> MNLLVTSSLGVLLHLVVLCQADDHSELLVNTKSGKVMGTRVPVLSSHISAFLGIPFAEPPVGNMRFRRPEPKKPWSGVWNASTYPNNCQQYVDEQFPGFSGSEMWNPNREMSE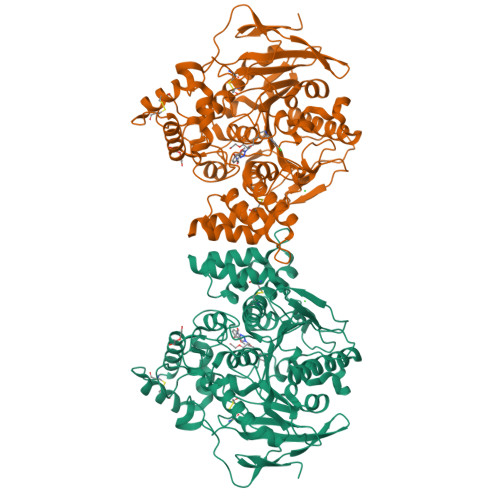DCLYLNIWVPSPRPKSTTVMVWIYGGGFYSGSSTLDVYNGKYLAYTEEVVLVSLSYRVGAFGFLALHGSQEAPGNVGLLDQRMALQWVHDNIQFFGGDPKTVTIFGESAGGASVGMHILSPGSRDLFRRAILQSGSPNCPWASVSVAEGRRRAVELGRNLNCNLNSDEELIHCLREKKPQELIDVEWNVLPFDSIFRFSFVPVIDGEFFPTSLESMLNSGNFKKTQILLGVNKDEGSFFLLYGAPGFSKDSESKISREDFMSGVKLSVPHANDLGLDAVTLQYTDWMDDNNGIKNRDGLDDIVGDHNVICPLMHFVNKYTKFGNGTYLYFFNHRASNLVWPEWMGVIHGYEIEFVFGLPLVKELNYTAEEEALSRRIMHYWATFAKTGNPNEPHSQESKWPLFTTKEQKFIDLNTEPMKVHQRLRVQMCVFWNQFLPKLLNATACDGELSSSGTSSSKGIIFYVLFSILYLIF6-chloro-2H-1,4-benzoxazin-3(4H)-one 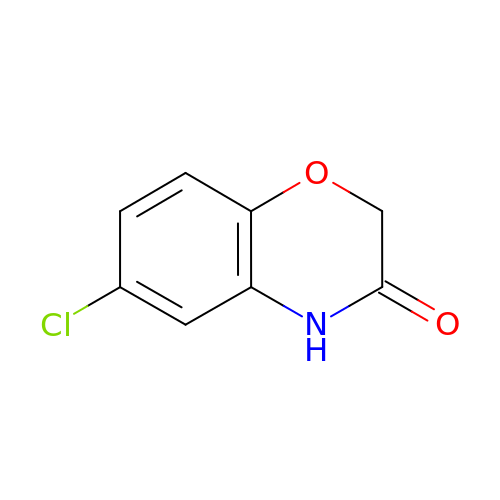| C8 H6 Cl N O2 | OBPIPKQQNRACHV-UHFFFAOYSA-N>[2x]GPGGSPYLITGIPKDPKHPLPIRKDIDDWYLEQTSAGSNRIQLTLFVEALTVIQNRPLNDQLSYFRLAGIHGAPWTEWDGVPGGQKDSKGNPTGFAVHNNYTFPTWFRVYVTLYEQVIYEAMLDFIKQNVPQNGKADWENEAKQWRLPYWDFARFARHGHDNTQGDELRLPILVTMPMVKVLVPGQPGKQLSKPNPLYRFQMQTLMGTLERPYAITSQKTEEHGWSFDLPFDKCQSTTKYGLLENYNADVWADGGQNWLRANLALNEHPWYQNLDGWDSVPTLQDMTFRLLTTGGLNWGEFSSTRYDDKKEETQPKNNEQAPKNWMNLEAIHNNVHNWVGGFMFSRPGRHDLKLWGAGHMSSVPVAAYDPIFWLHHCNIDRLTAIWQTVNSGSWFNDDKSKVSKDDDLRPFHRFCEKTRKVVFFRSDDV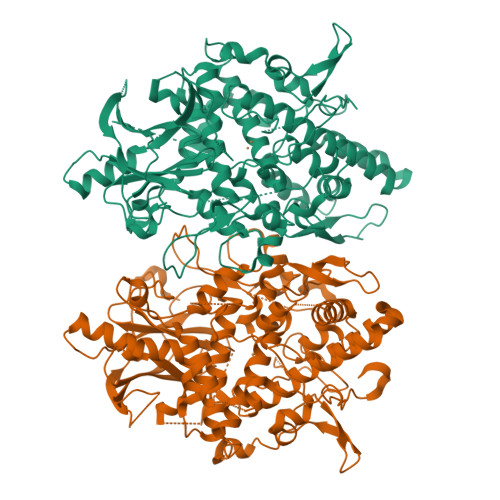KDWRSLNYDYAITKDASRIRKEISDLYGQRTKEVYKDFGEEDYILSIRYSRYALGGKPFQINIFFGDVDGKDFYDARSQNFVGSVFNFSGSLEDSNCDKCAQQEQEGVLSVSQLPARLAVHYYKKQNKGEVPTPRYVVVNSQGKAEAEVKVEVALHKTEGTFYDAPARGGSDDYRRVADGKRAEVDDAYRA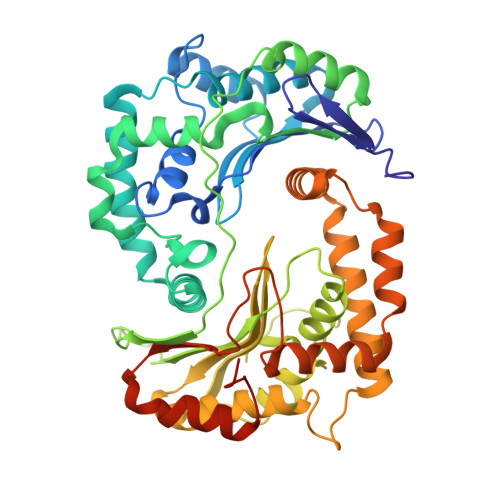> ARTDNFKLSSLANGLKVATSNTPGHFSALGLYIDAGSRFEGRNLKGCTHILDRLAFKSTEHVEGRAMAETLELLGGNYQCTSSRENLMYQASVFNQDVGKMLQLMSETVRFPKITEQELQEQKLSAEYEIDEVWMKPELVLPELLHTAAYSGETLGSPLICPRGLIPSISKYYLLDYRNKFYTPENTVAAFVGVPHEKALELTGKYLGDWQSTHPPITKKVAQYTGGESCIPPAPVFGNLPELFHIQIGFEGLPIDHPDIYALATLQTLLGGGGSFSAGGPGKGMYSRLYTHVLNQYYFVENCVAFNHSYSDSGIFGISLSCIPQAAPQAVEVIAQQMYNTFANKDLRLTEDEVSRAKNQLKSSLLMNLESKLVELEDMGRQVLMHGRKIPVNEMISKIEDLKPDDISRVAEMIFTGNVNNAGNGKGRATVVMQGDRGSFGDVENVLKAYGLGNSSSSKNDSPKKKGWFHHHHHH>[2x]APRKFFVGGNWKMNGDKKSLGELIHTLNGAKLSADTEVVCGAPSIYLDFARQKLDAKIGVAAQNCYKVPKGAFTGEISPAMIKDIGAAWVILG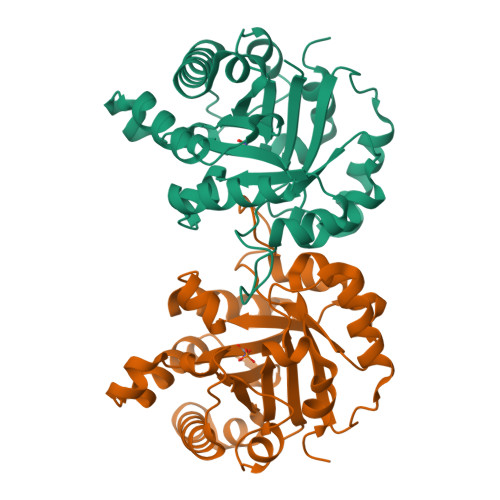NSERRHVFGESDELIGQKVAHALAEGLGVIACIGEKLDEREAGITEKVVFEQTKAIADNVKDWSKVVLAYEPVWAIGTGKTATPQQAQEVHEKLRGWLKTHVSDAVAQSTRIIYGGSVTGGNCKELASQHDVDGFLVGGASLKPEFVDIINAKH>[4x]MKVAPAPASGQPGGGSKKPSDYGCQLHYKHARVVEPESTTDDGMKRLKDVGDKGTLITAAELGLVDKYRDLKRAGQDILTCDWPYHYS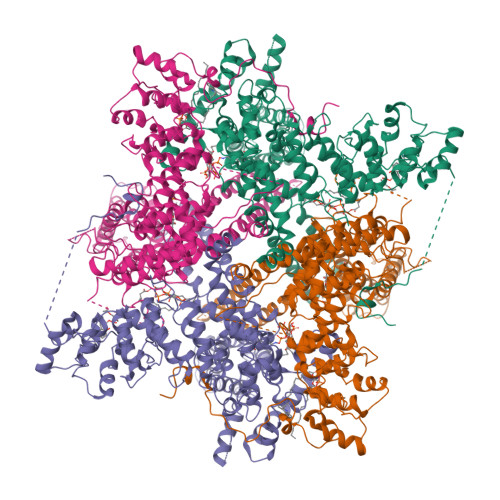SILYACYGNQYKILQMVEREFVGSTQELTAMHTTRCWVGKNSAMVAAYQGHLETMLYIIDLDMQGKFTEDLFKQRDVMGKNAMMWAASQGHTDTIEVLLVRSLYRLLPEDCADPLVLKTRWKLVSLLADLASHCRDYDPGCSRSFFQEVLASIKYDPVEGARQEEAAAAGGGGSAREGAALHEPTWGVDDGEEEERRHGVKHSDLVGKSAASTTAAAAAGGKTASGKPGEPGGGGAVKLKDVHITVRTLQGVIVSAYRAGMNCMGVIMYCQSLLQQARYFDDLVAQLTAWEVKLLDTCRNKQEVQAILAPTEDDPSEPVGYALATFDKAFLSHKFVQQIFTEKWDTMGVTDYTKSLFGVVWGGCSLVVAFAAWATICPLVVVARSFLSPVQDFMMRGKVIVDSRFPWHVPLYRWLLTQCALITFTVLLSYLVFSFDPSDPVPASVAPLNTFLAVWCAAILVDEVQEYVEEGRAEYMSSGWNVMDVTMALSYILHYILRIIAVRVTDNLNILLVVNDLLAAAALMAWFRMVSVFELSSAIGPLIQMMKQMLIKDVTRFALLVLVILLGFSVGMEALFQEACIERDPTTNECTKYTSWGYDWQKDGLVGGMTFLQYIALGNANPVDFEQKRVTGVIFYLIFAIVTAILLLNLFIAMLADTYTRVSTQAMVEFRYRKAKLMASYSRRDFVCPPFNLLHLVCAAVGNGLRRLVWGPDGFTPVSMRKNETVPLFSWYFPQGEEMRQVVVLQRRVVDDFLNSNRVALFREKLNAELPNLVHEMLKQKGKGDGGALAGGGAAASTTVLATAVSVTAAAGH>[2x]GDPYWAYSGAYGPEHWVTSSVSCGGRHQSPIDILDQYARVGEEYQELQLDGFDNESSNKTWMKNTGKTVAILLKDDYFVSGAGLPGRFKAEKVEFHWGHSNGSAGSEHSINGRRFPVEMQIFFYNPDDFDSFQ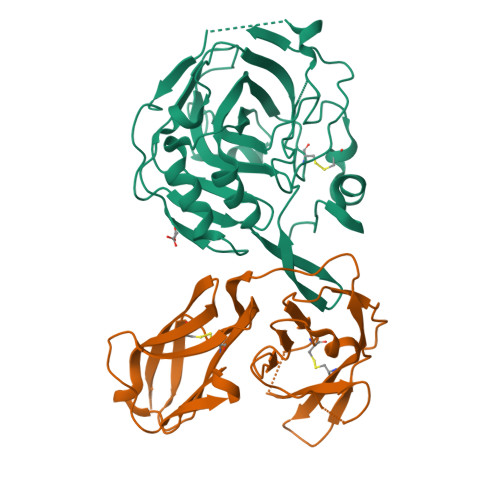TAISENRIIGAMAIFFQVSPRDNSALDPIIHGLKGVVHHEKETFLDPFVLRDLLPASLGSYYRYTGSLTTPPCSEIVEWIVFRRPVPISYHQLEAFYSIFTTEQQDHVKSVEYLRNNFRPQQRLHDRVVSKS;>FKTRMRSTVSVREGQGVVLLCGPPPHSGELSYAWVFNEYPSFVEEDSRRFVSQETGHLYIAKVEPSDVGNYTCVVTSTVTNTRVLGSPTPLVLRSDGVMGEYEPKIEVQFPETLPAAKGSTVRLECFALGNPVPQINWRRSDGMPFPNKIKLRKFNGMLEIQNFQQEDTGSYECIAENSRGKNVARGRLTYYA[2x]> MEHRAFKWPQPLAGNKPRIWYGGDYNPDQWPEEVWDEDVALMQQAGVNLVSVAIFSWAKLEPEEGVYDFDWLDRVIDKLGKAGIAVDLASGTASPPMWMTQAHPEILWVDYRGDVCQPGARQHWRATSPVFLDYALNLCRKMAEHYKDNPYVVSWHVSNEYGCHNRFDYSEDAERAFQKWCEKKYGTIDAVNDAWGTAFWAQRMNNFSEIIPPRFIGDGNFMNPGKLLDWKRFSSDALLDFYKAERDALLEIAPKPQTTNFMVSAGCTVLDYDKWGHDVDFVSNDHYFSPGEAHFDEMAYAACLTDGIARKNPWFLMEHSTSAVNWRPTNYRLEPGELVRDSLAHLAMGADAICYFQWRQSKAGAEKWHSAMVPHAGPDSQIFRDVCELGADLNKLADEGLLSTKLVKSKVAIVFDYESQWATEHTATPTQEVRHWTEPLDWFRALADNGLTADVVPVRGPWDEYEAVVLPSLAILSEQTTRRVREYVANGGKLFVTYYTGLVDDRDHVWLGGYPGSIRDVVGVRVEEFAPMGTDAPGTMDHLDLDNGTVAHDFADVITSVADTAHVVASFKADKWTGFDGAPAITVNDFGDGKAAYVGARLGREGLAKSLPALLEELGIETSAEDDRGEVLRVERADETGENHFVFLFNRTHDVAVVDVEGEPLVASLAQVNESEHTAAIQPNGVLVVKLAAALEHHHHHH

Aim: Bifidobacterium longum subsp. infantis uses a glycoside hydrolase (GH) family 42 β-galactosidase (BiBga42A) for hydrolyzing lacto-N-tetraose (LNT), which is the most abundant core structure of human milk oligosaccharides (HMOs). As such, BiBga42A represents one of the pivotal enzymes underpinning the symbiosis between bifidobacteria and breastfed infants. BiBga42A has a three-dimensional structure similar to other GH42 enzymes that have three domains consisting of a (β/α)8 barrel (domain A), an α/β fold (domain B), and an anti-parallel β-sandwich (domain C). Glu-160 and Glu-318 in BiBga42A were predicted to be the acid/base catalyst and the nucleophile, respectively, based on previous studies of GH42 enzymes and sequence alignment.

First, we determined the structure of the WT enzyme complexed with glycerol (WT-GOL) at 1.7 Å resolution. The electron density of a glycerol molecule, which was used as a cryoprotectant, was observed at the active site, even though the crystals were grown in the presence of Gal. The asymmetric unit of the WT-GOL crystal contained one molecule of BiBga42A, and it forms a homotrimer with symmetry-related molecules by a crystallographic 3-fold axis. A PISA molecular interface analysis calculated that approximately 27% of the entire surface area of the trimer (17,082 Å of 64,278 Å) was buried. Our previous study using calibrated gel filtration chromatography also suggested that BiBga42A forms a trimer in solution. The trimeric structure of BiBga42A resembles a flowerpot, like other GH42 enzymes[23-25]. The glycerol molecule in WT-GOL occupies the C2-C4 position of the Gal.>ADKLPNIVILATGGTIAGSAATGTQTTGYKAGALGVDTLINAVPEVKKLANVKGEQFSNMASENMTGDVVLKLSQRVNELLARDDVDGVVITHGTDTVEESAYFLHLTVKSDKPVVFVAAMRPATAISADGPMNLLEAVRVAGDKQSRGRGVMVVINDRIGSARYITKTNASTLDTFRANEEGYLGVIIGN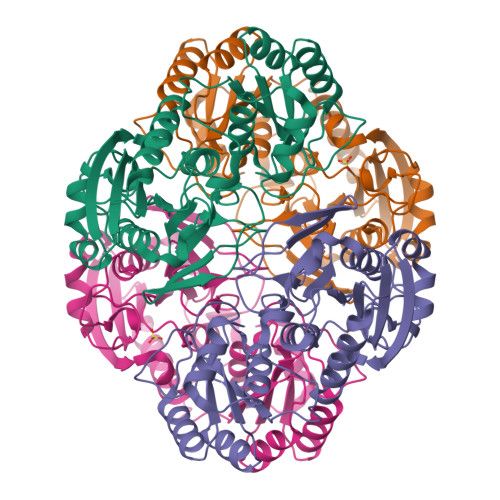RIYYQNRIDKLHTTRSVFDVRGLTSLPKVDILYGYQDDPEYLYDAAIQHGVKGIVYAGMGAGSVSVRGIAGMRKALEKGVVVMRSTRTGNGIVPPDEELPGLVSDSLNPAHARILLMLALTRTSDPKVIQEYFHTY[2x]> SGRPSTDALKLCPHEEFLRLCKERAEEIYPIKERNNRTRLALIICNTEFDHLPPRNGADFDITGMKELLEGLDYSVDVEENLTARDMESALRAFATRPE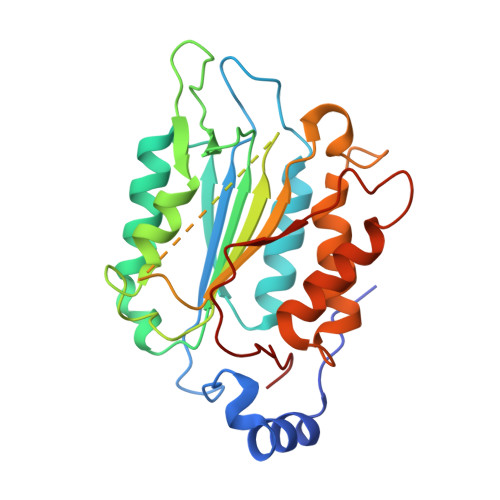HKSSDSTFLVLMSHGILEGICGTVHDEKKPDVLLYDTIFQIFNNRNCLSLKDKPKVIIVQAARGANRGELWVRDSPASLEVASSQSSENLEEDAVYKTHVEKDFIAFCSSTPHNVSWRDSTMGSIFITQLITCFQKYSWCCHLEEVFRKVQQSFETPRAKAQMPTIERLSMTRYFYLFPGN Here, we study the kinetics and substrate specificity of an AldDH enzyme from the Clostridium phytofermentans fucose/rhamnose utilisation BMC, Cphy1178. The overall structure corresponds to other members in the aldehyde dehydrogenase family, with a catalytic domain (residues 238–427, highlighted pink), a cofactor-binding domain with the Rossman-fold type nucleotide binding architecture (residues 28–108, 127–237, and 428–447, highlighted grey), and an oligomerisation domain (residues 109–126 and 448–462, highlighted green). The catalytic and nucleotide binding domains come together to form an extended nucleotide and ligand-binding tunnel that is open at both ends, with the catalytic cysteine (C269) at the centre of the tunnel and the NAD+ cofactor binding at one side. Cphy1178 forms a tetrameric quaternary structure generated by crystal symmetry, with molecules related by D2 symmetry.

The structures of Cphy1178 were also solved with mutations in active site residues, C269A with bound CoA (1.77 Å resolution) and H387A (2.08 Å resolution) to ensure that mutation of these residues did not destabilise the structure of the protein. Both of these proteins display essentially identical structures to the wild-type protein. Mutagenesis of a strictly conserved Histidine residue (H387), that is within 2.5 Å of the catalytic cysteine completely abolishes activity of the enzyme. This residue is not found in any of the non-acylating aldehyde dehydrogenase enzymes. The proximity of this residue to the catalytic cysteine is incompatible with the formation of the correct geometry for deprotonation of water for resolution of the acyl-intermediate to produce a carboxylic acid product. In light of our biochemical data showing that the H387A mutant is inactive, we suggest that this residue acts as a base to activate the catalytic cysteine and to stabilise the acyl-transfer intermediate between the enzyme and CoA cofactor. In our reaction scheme H387 deprotonates the catalytic cysteine to allow nucleophilic attack on the substrate to form tetrahedral intermediate.

> MGQLTQTNKTELGVFDDMNQAIEAAKEAQLVVKKMSMDQREKIISAIRKKTIEHAETLARMAVEETGMGNVGHKILKHQLVAEKTPGTEDITTTAWSGDRGLTLVEMGPFGVIGAITPCTNPSETIICNTIGMLAGGNTVVFNPHPAAIKTSNFAVQLINEASLSAGGPVNIACSVRKPTLDSSKIMMSHQDIPLIAATGGPGVVTAVLQSGKRGIGAGAGNPPVLVDETADIRKAAEDIINGCTFDNNLPCIAEKEVVAIDAIANELMNYMVKEQGCYAITKEQQEKLTNLVITPKGLNRNCVGKDARTLLGMIGIDVPSNIRCIIFEGEKEHPLISEELMMPILGIVRAKSFDDAVEKAVWLEHGNRASAHIHSKNVDRITTYAKAIDTAILVKNAPSYAAIGFGGEGFCTFTIASRTGEGLTSASTFTKRRRCVMSDSLCIR> VETISFSFSEFEPGNDNLTLQGAALITQSGVLQLTKINQNGMPAW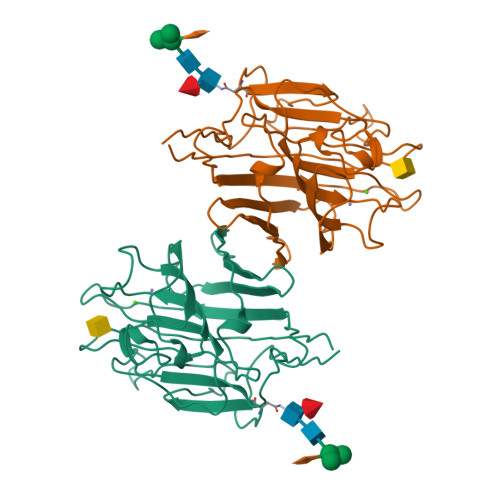DSTGRTLYAKPVHIWDMTTGTVASFETRFSFSIEQPYTRPLPADGLVFFMGPTKSKPAQGYGYLGIFNNSKQDNSYQTLGVEFDTFSNPWDPPQVPHIGIDVNSIRSIKTQPFQLDNGQVANVVIKYDASSKILHAVLVYPSSGAIYTIAEIVDVKQVLPEWVDVGLSGATGAQRDAAETHDVYSWSFQASLPE> MGSYLHEPPGDEPSMRIEQPKTADRAPEQVAIHICEPSKVVTESFPFSETAEPEAKSKNCPCPEIARIGPCPNKPPKIPINRGLSRISTNKSRPKSRFGEPSWPVESSLDLTSQSPVSPYREEAFSVENCGTAGSRRGSFARGTTSRAASSSRKDETKEGPDEKEVYQRVTAQLSARNQKRMTVKLMIELSVFLCLLGCLVCSLTVDGFKRYTVIGLDIWKWFLLLLVIFSGMLITHWIVHVAVFFVEWKFLMRKNVLYFTHGLKTSVEVFIWITVVLATWVMLIKPDVNQPHQTRKILEFVTWTIVTVLIGAFLWLVKTTLLKILASSFHLNRFFDRIQESVFHHSVLQTLAGRPVVELAQGISRTESQDGAGQVSFMEHTKTQNKKVVDVGKLHQMKQEKVPA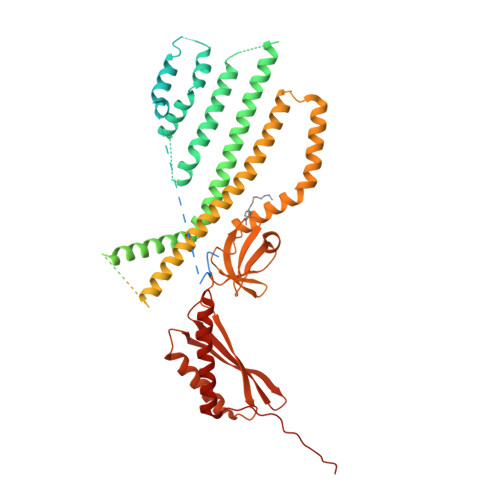WTMQLLVDVVSNSGLSTMSGMLDEDMVEGGVELDDDEITNEEQAIATAVRIFDNIVQDKVDQSYIDRVDLHRFLIWEEVDHLFPLFEVNEKGQISLKAFAKWVVKVYNDQAALKHALNDNKTAVKQLNKLVTAILIVMMIVIWLIVTGIATTKLIVLLSSQLVVAAFIFGNTCKTIFEAIIFVFVMHPFDVGDRCVIDGNKMLVEEMNILTTVFLKWDKEKVYYPNSILCTKAIGNFFRSPDQGDVLEFSVDFTTPVLKIGDLKDRIKMYLEQNLNFWHPQHNMVVKEIENVNKIKMALFVNHTINFQDFAEKNRRRSELVLELKKIFEELDIKYNLLPQEISIRNMGSGSLEVLFQ> MSELLIKNGYIFDPISGIKGDKADIAIKDGKIVDKVSSKAQVIDASGKTVMSGGVDIHTHVSGPKVNTGRMMRPEDKFFRGSYRGGIIKQGKRMEMGFSIPSTYKTGYAYARMGYTFTNEAAMPPLLAPHVHEEFRDTPILDQAAMPVFGNNWFCFEYIKNKELENNAAYVAWLLNATKGIGIKVVNPGGTEAWAWGENCTTINDPVPYFDITPAEIVKGLIETNEYLGLPHSVHIHG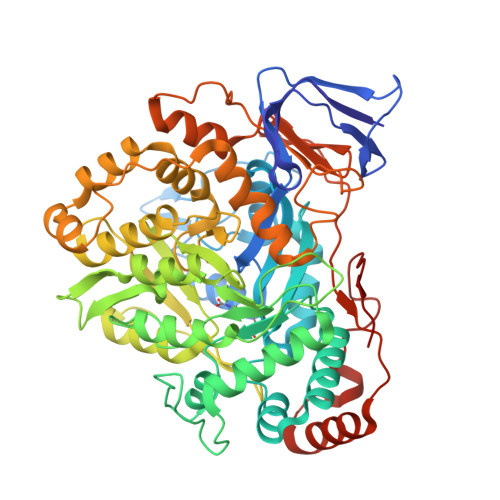NNLGNPGNYKDTLDTLRLAESYKAKNKFGREQVLHNTHIQFHSYKGTSWADFESGAKEIMDYVNANKNITCDIGQVTLDETTTMTADGPFEYHLNQLNHIKWANVDVELETGSGVVPYIYDKNIKVCGIQWAIGLELALYAKDLMRVHITTDHPNAGPFTRYPCVIKWLMSEKARKATLDTMKWKDKVIAASNIASMDRELGLYEIAMMTRAGPAKALGLAAIYGSLVKGADGNVAIYNLDANDLPSDPELIEAAFQNTAYTIKEGVVVVKDGEIIAEPHKYTLWTKVNMPENAQVMHDIKEKFTKNYTVNLENYAVFDEHVHNPRAIELDVA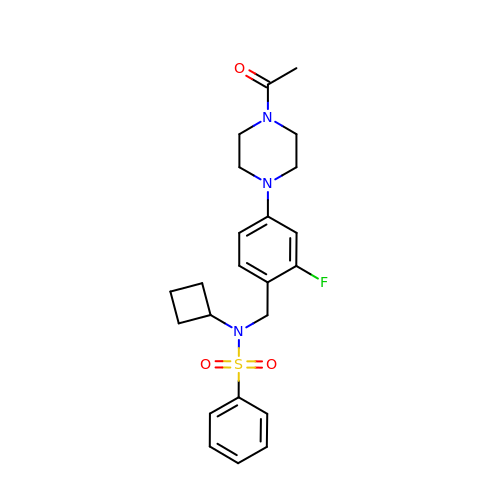N-[4-(4-acetylpiperazin-1-yl)-2-fluorobenzyl]-N-cyclobutylbenzenesulfonamide | C23 H28 F N3 O3 S | PIGCNHMXDYACOO-UHFFFAOYSA-N>[2x]VAWYARYPHILEEATRLPFAYPIGQYYDTGYSVASATEWSKYVDTSLTIPGVMCVNFTPTPGESYNKNSPINIAAQNVYTYVRHMNSGHANYEQADLMMYLLAMDSLYIFHSYVRKILAISKLYTPVNKYFPRALLVALGVDPEDVFANQAQWEYFVNMVAYRAGAFAAPASMTYYERHAWMSNGLYVDQDVTRAQIYMFKPTMLWKYENLGTTGTKLVPLMMPKAG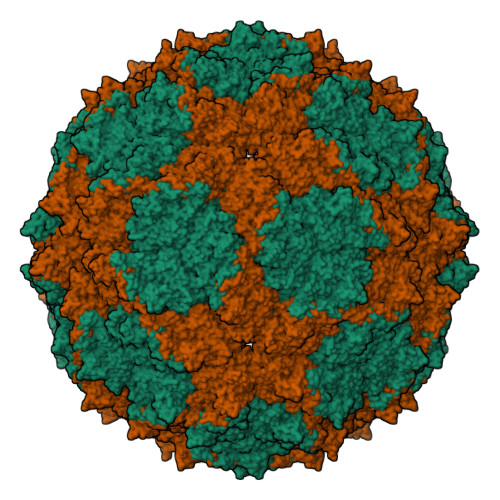DNRKLVDFQVLFNNLVSTMLGDEDFGIMSGDVFKAFGADGLVKLLAVDSTTMTLPTYDPLILAQIHSARAVGAPILETSTLTGFPGRQWQITQNPDVNNGAIIFHPSFGYDGQDHEELSFRAMCSNMILNLPGEAHSAEMIIEATRLATMFQVKAVPAGDTSKPVLYLPNGFGTEVVNDYTMISVDKATPHDLTIHTFFNNILVPNAKENYVANLELLNNIIQFDWAPQLYLTYGIAQESFGPFAQLNDWTILTGETLARMHEVCVTSMFDVPQ> MKAEIKNLIDRGTYRKLPLFEGELPEGSYAQIVEVKPKQTVKKHYHERQYELFYIISGEARLGIGDTEYQAKPGDIFLVKPKTVHWVVNEKDEPFRLFVVKLNYHGDDSVWLE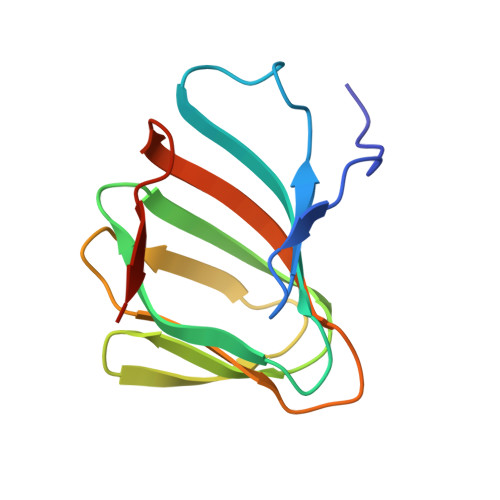GSF> GGUUGCCGAAUCCAUGAUUUGGUACGGAGGAACCGCUUUUUGGGGUUAAUCUGCAGUGAAGCUGCAGUAGGGAUACCUUCUGUCCCGCAC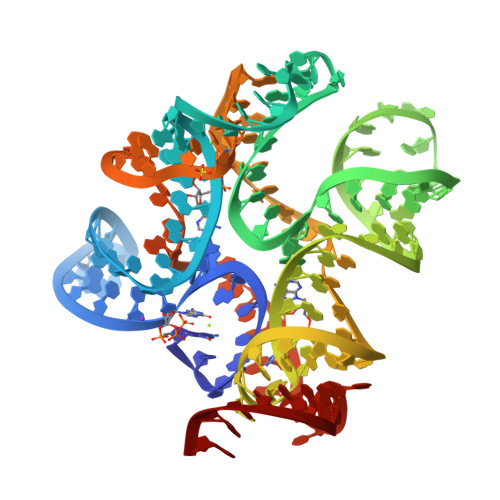CCGACAGCUAACUCCGGAGGCAAUAAAGGAAGGAG> GRKSVPCGWERVVKQRLFGKTAGRFDV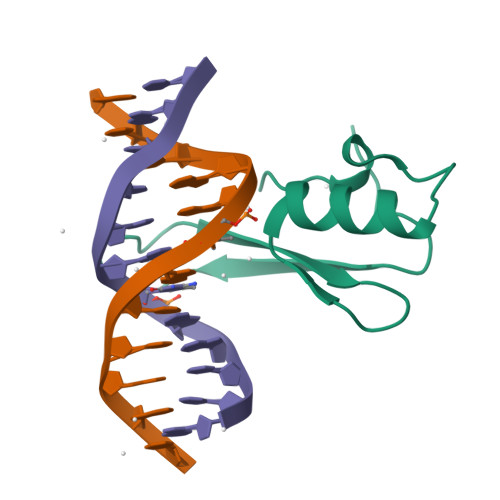YFISPQGLKFRSKSSLANYLHKNGETSLKPEDFDFTVLSKR> RWWTRASGMRNPVKWTRDWEVLNRKVYFAFDEREIRRSMLDAVNAHRKTASLFHRMINAVPGVAHAMSLPGPHTFFLPSDKACRDHLSPDSLHALTERVAFLEEQQRQRVGARVQVEGGVSVRGGTAAAIADRVAKTTEQLRTFVLAHLIPGEWRMKTLLLACGAGDPRRNGSLRYQDT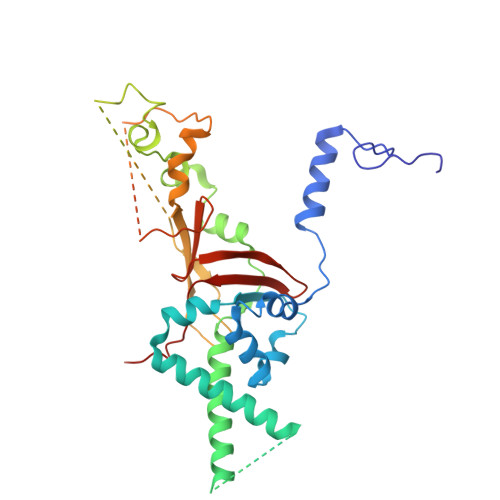DRELFAPVMYASRLGTGEKTKRRQTASREGVEHENAQELGRTRDEETDRSSVFLLPPPQSTDEPLPVWVQASRYAAFLPITTSTNFPRFEGTECRGNSDREEAESVENSGEYSQRRSTVGGALHLWVGGALVTKGDLRAHNGVVHMIDKPLIPVQLLAS The mono-ubiquitination of the histone protein H2B (H2Bub1) is a highly conserved histone post-translational modification that plays critical roles in many fundamental processes. In the budding yeast, the H2Bub1 reaction is catalyzed by the E3 enzyme Bre1 together with the E2 enzyme Rad6. In addition to the RING domain, Bre1 contains a N-terminal Rad6-binding domain (RBD) that also makes important contributions to the H2Bub1 catalysis. We found that the interaction stimulates Rad6’s enzymatic activity by allosterically increasing its active site accessibility and likely contribute to the H2Bub1 catalysis through additional mechanisms.

We screened through several fungal species and were able to crystallize the Kluyveromyces lactis Rad6 (KlRad6) in complex with the Kluyveromyces lactis Bre1 (KlBre1) N-terminal fragment 1-206 or 1-184 (crystal forms 1 and 2, respectively). The structures were refined to resolutions of 3.2 and 3.05 Å. The complexes in both crystal forms adopt similar conformations, except for complex 1 in crystal form 2. The orientation of KlRad6 in this complex is related to the orientation of KlRad6 in other complexes by a rotation of 14°. KlRad6 in this complex forms extensive interactions with neighboring protein molecules in the crystal, which may play a role in stabilizing the observed structure. In contrast, KlRad6 molecules in the other three complexes do not mediate extensive crystal packing interactions. When the three KlRad6 molecules not mediating extensive crystal packing interactions in our structures are compared, large structural differences are observed for residues 90–98 and 115–121 surrounding KlRad6’s active site. The 90–98 region can be resolved in the electron density map in crystal form 1 but is mostly disordered in KlRad6 molecule 2 in crystal form 2, the equivalent Cα atoms in the 115–121 region are located as far as 5.2 Å apart. In contrast, in KlRad6 molecule 1 in crystal form 2, the temperature factors for these regions are not elevated, consistent with stabilization of their structure by the extensive crystal packing interactions.

>[2x]GSHMSTPARRRLMRDFKRMKEDSPPGVSASPLPDNVMIWNAMIIGPADTPYEDGTFRLLLEFDEEYPNKPPHVKFLSEMFHPNVYANGEICLDILQNRWTPTYDVASILTSIQSLFNDPNPASPANVEAATLFQDHKSQYVKRVKETVEKSWEDDMEDMADEDEDEE;>[4x]MNDHFVKRPKLELSDPSEPLTQKDVIAFQKEALFRCLNKWRVKANQLVEENEVLAAGLSKTTESVSGCCSSIVVLARSVVEDCSDEQDKRFLQQLINTEDEHTLTQIISNNSARICELILKTSGSNISDNIGRLQELESLTLTLQKLLKSSENKLKKATEYYENIIAQYDRQDSESVSRVFNTADDDSNVKKEKQSSTGASSVNDE> XEDMTHVPTDAFGKLERPAAVFNHDEHNEKAGIESCNACHHVWVNGVLAEDEDSVGTPCSDCHALEQDG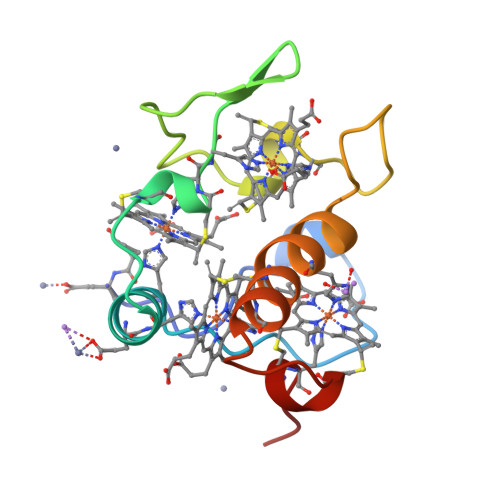DTPGLQDAYHQQCWGCHEKQAKGPVMCGECHVKN>[2x]GNSVTYTTLISGLGKAGRLEEALELFEEMKEKGIVPDVVTYTTLISGLGKAGRLEEALELFEEMKEKGIVPDVVTYTTLISGLGKAGRLEEALELFEEMKEKGIVPDVVTYTTLISGLGKAGRLEEALELFEEMKEKGIVPDVVTYT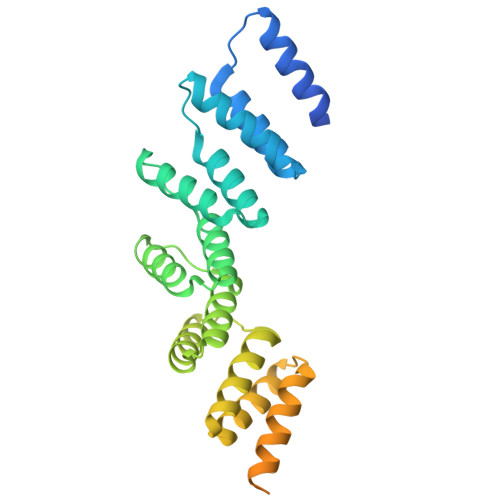TLISGLGKAGRLEEALELFEEMKEKGIVPDVVTYTTLISGLGKAGRLEEALELFEEMKEKGIVPDVVTYTTLISGLGKAGRLEEALELFEEMKEKGIVPDVVTYTTLISGLGKAGRLEEALELFEEMKEKGIVPDVVTYTTLISGLGKAGCGRALE>MKFSVIVPTYNSEKYITELLNSLAKQDFPKTEFEVVVVDDCSTDQTLQIVEKYRNKLNLKVSQLETNSGGPGKPRNVALKQAEGEFVLFVDSDDYINKETLKDAAAFIDEHHSDVLLIKMKGVNGRGVPQ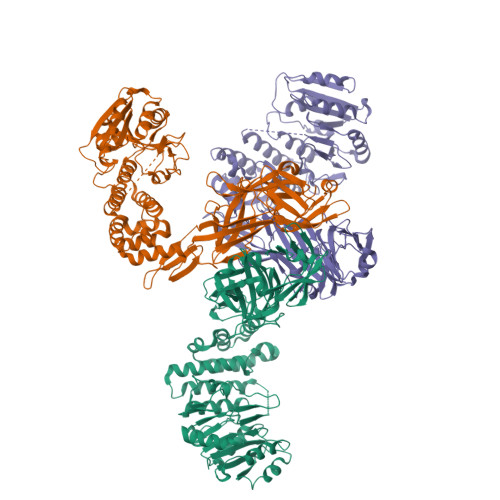SMFKETAPEVTLLNSRIIYTLSPTKIYRTALLKDNDIYFPEELKSAEDQLFTMKAYLNANRISVLSDKAYYYATKREGEHMSSAYVSPEDFYEVMRLIAVEILNADLEEAHKDQILAEFLNRHFSFSRTNGFSLKVKLEEQPQWINALGDFIQAVPERVDALVMSKLRPLLHYARAKDIDNYRTVEESYRQGQYYRFDIVDGKLNIQFNEGEPYFEGIDIAKPKVKMTAFKFDNHKIVTELTLNEFMIGEGHYDVRLKLHSRNKKHTMYVPLSVNANKQYRFNIMLEDIKAYLPKEKIWDVFLEVQIGTEVFEVRVGNQRNKYAYTAETSALIHLNNDFYRLTPYFTKDFNNISLYFTAITLTDSISMKLKGKNKIILTGLDRGYVFEEGMASVVLKDDMIMGMLSQTSENEVEILLSKDIKKRDFKNIVKLNTAHMTYSLK[3x]1-(1-METHYLETHYL)-3-(PYRIDIN-3-YLETHYNYL)-1H-PYRAZOLO[3,4-D]PYRIMIDIN-4-AMINE | C15 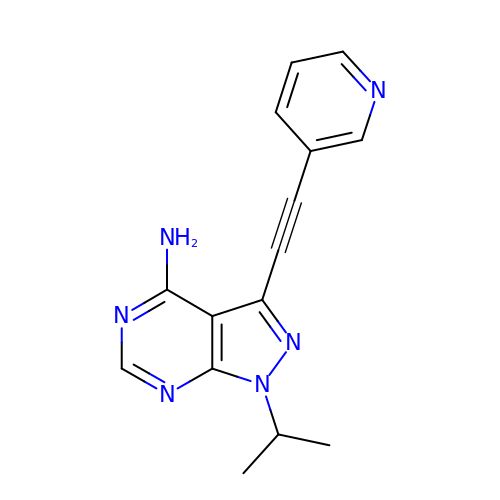H14 N6 | NYVMTNNWZOHTJT-UHFFFAOYSA-N> GQRGWFCGSVSQDLRQFWVAEGGTISDPRAADFLFSCDASHPDTLRIYQSLDYIEDNATVFHAYYLSAVANAKIKNSVALGHFILPPACLQKEIRRKIGSFIWEQDQ;> YRCSGCIAVEKSLNSRNFSKLLHSCPYQCDRHKVIVEAEDRYK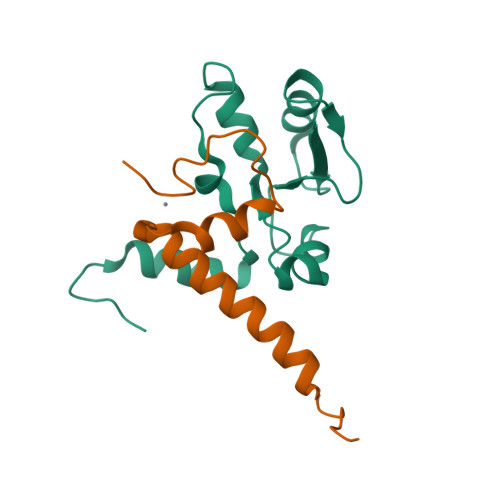SELRKSLICNKKILLTP>CGLVASNLNLKPGECLRVRGEVAPDAKSFVLNLGKDSNNLCLHFNPRF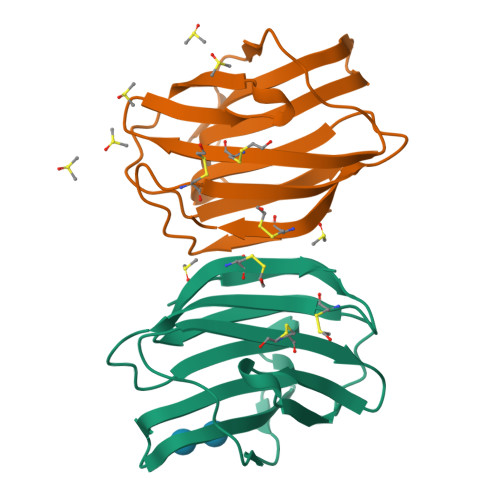NAHGDANTIVCNSKDGGAWGTEQREAVFPFQPGSVAEVCITFDQANLTVKLPDGYEFKFPNRLNLEAINYMAADGDFKIKCVAFD[2x]(3S)-citryl-Coenzyme A | C27 H42 N7 O22 P3 S 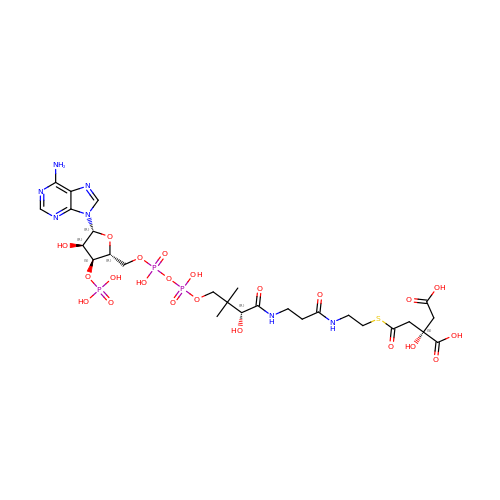| IHVFHZGGMJDGGZ-VPXVXCNZSA-N>[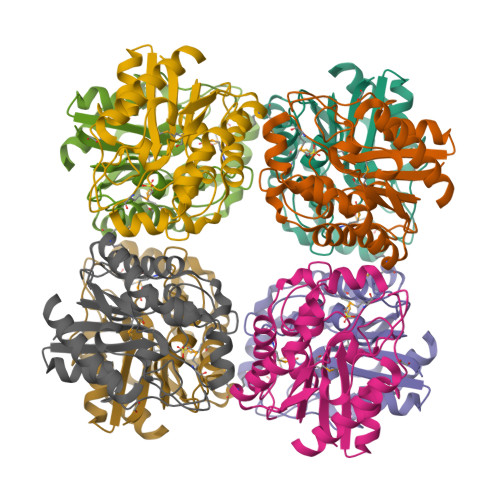8x]MAKRILCFGDSLTWGWVPVEDGAPTERFAPDVRWTGVLAQQLGADFEVIEEGLSARTTNIDDPTDPRLNGASYLPSCLATHLPLDLVIIMLGTNDTKAYFRRTPLDIALGMSVLVTQVLTSAGGVGTTYPAPKVLVVSPPPLAPMPHPWFQLIFEGGEQKTTELARVYSALASFMKVPFFDAGSVISTDGVDGIHFTEANNRDLGVALAEQVRSLL>SVKLAGNSSLCPVSGWAIYSKDNSVRIGSKGDVFVIREPFISCSPLECRTFFLTQGALLNDKHSNGTIKDRSPYRTLMSCPIGEVPSPYNSRFESVAWSASACHDGINWLTIGISGPDNGAVAVLKYNGIITDTIKSWRNNVLRTQESECACVNGSCFTVMTDGPSNGQASYKIFRIEKGKIVKSVEMNAPNYYYEECSCYPDSSEITCVCRDNWHGSNRPWVSFNQNLEYQIGYICSGIFGDNPRPNDKTGSCGPV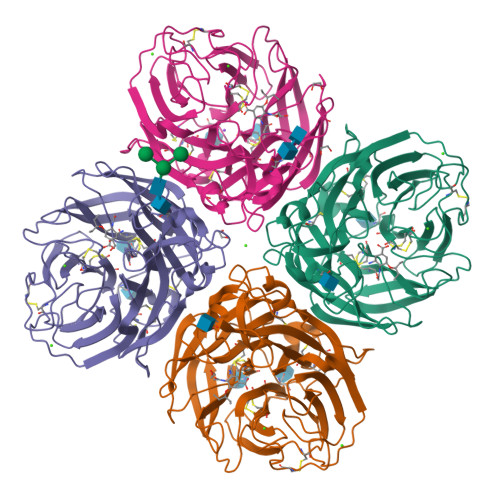SSNGANGVKGFSFKYGNGVWIGRTKSISSRNGFEMIWDPNGWTGTDNNFSIKQDIVGINEWSGYSGSFVQHPELTGLDCIRPCFWVELIRGRPKENTIWTSGSSISFCGVNSDTVGWSWPDGAELPFTIDK[4x]> MRGSHHHHHHGSMGKGITGFDPSLYSYLQSISADDSFYLAQLRRETAHLPGAPMQISPEQAQFLGLLISLTGAKQVLEIGVF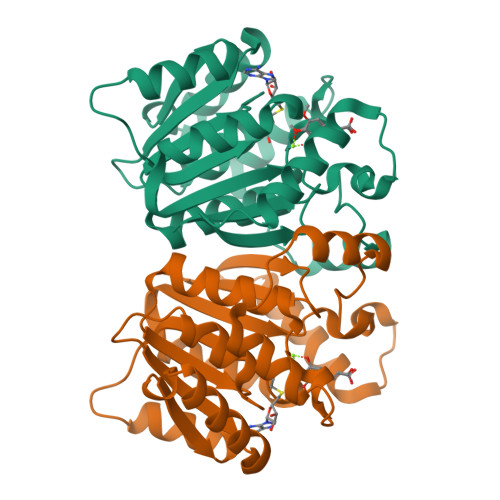RGYSALAMALQLPPDGQIIACDQDPNATAIAKKYWQKAGVAEKISLRLGPALATLEQLTQGKPLPEFDLIFIDADKRNYPRYYEIGLNLLRRGGLMVIDNVLWHGKVTEVDPQEAQTQVLQQFNRDLAQDERVRISVIPLGDGMTLALKK(2R,3R,4R,5R)-4,5-dihydroxy-2-(hydroxymethyl)-6-oxopiperidin-3-yl 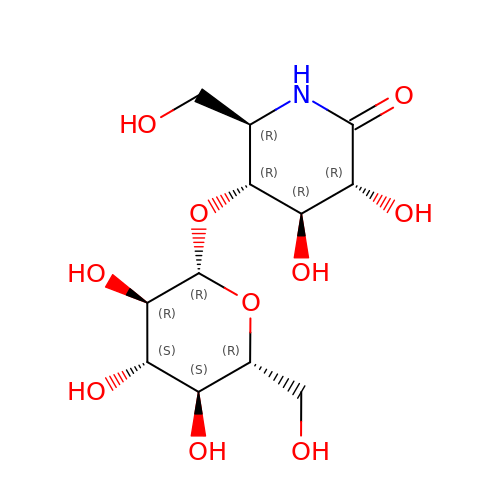beta-D-glucopyranoside | C12 H21 N O10 | WXSNJJDPPISYEF-ZNLUKOTNSA-N TRPV4 is a polymodal, calcium-permeable cation channel that has emerged as a potential therapeutic target in multiple conditions. TRPV4, expressed in the plasma membrane of a wide range of cell types, is a polymodal ion channel whose gating is controlled by multiple endogenous lipids, and exogenous stimuli including synthetic ligands, cell swelling, shear stress, moderate heat, and ultraviolet light. Human TRPV4 adopts a two-layered homotetrameric architecture where RhoA attaches to the bottom layer. RhoA appears to act as an auxiliary subunit, interacting with the ARD through three loops connecting AR2-AR3, AR3-AR4, AR4-AR5, and with the membrane bilayer through the prenylated C-terminal tail.

Particle subtraction followed by focused 3D classification of the transmembrane region and RhoA-bound cytoplasmic domain were performed, resulting in improved map qualities for these regions for model building. In our ligand-bound 3D cryo-EM reconstructions, we identified strong and unambiguous EM densities corresponding to GSK279 (antagonist), GSK101 (agonist), and 4α-PDD (agonist) located at a shared site within the cavity between the VSLD and the TRP domain (termed here the VSLD cavity). We functionally probed the interactions of GSK101 with TRPV4 by mutating amino acid residues within the GSK101 binding site using patch clamp recording on HEK293 cells expressing WT as well as mutant TRPV4. Mutations Y553A, N474A, and F524A significantly increased EC50 values of GSK101 for TRPV4, consistent with observations from the structural analysis. The GSK101 binding pose remained stable during the simulations, supporting its accuracy. However, in the GSK101-bound open state, the SF and the PHs move closer to enable cation coordination (the diagonal distance of G679 backbone carbonyl is 7.0 Å), which is consistent with previous mutagenesis studies. Meanwhile the pore-lining S6 helices rotate ~90°, thus changing the gate position (from M718 to I715) and the gate opening (the diagonal distance at I715 is 8.3 Å). This S6 rotation between the two states is due to the shift of the π-helix position on S6, resulting in a local secondary structure conversion between α- and π-helix along S6b, which is unique amongst the TRP channels. To validate the S6 gate position observed in the open-state structure, we performed Cd2+-dependent blocking of TRPV4. Among cysteine mutants near the S6 gate (I715C, A716C, L717C, and M718C), only I715C showed substantial inhibition of GSK101-elicited current by extracellular Cd2+, supporting the observation that I715 faces the ion permeation pathway in the TRPV4 open state.

>[4x]MADSSEGPRAGPGEVAELPGDESGTPGGEAFPLSSLANLFEGEDGSLSPSPADASRPAGPGDGRPNLRMKFQGAFRKGVPNPIDLLESTLYESSVVPGPKKAPMDSLFDYGTYRHHSSDNKRWRKKIIEKQPQSPKAPAPQPPPILKVFNRPILFDIVSRGSTADLDGLLPFLLTHKKRLTDEEFREPSTGKTCLPKALLNLSNGRNDTIPVLLDIAERTGNMREFINSPFRDIYYRGQTALHIAIERRCKHYVELLVAQGADVHAQARGRFFQPKDEGGYFYFGELPLSLAACTNQPHIVNYLTENPHKKADMRRQDSRGNTVLHALVAIADNTRENTKFVTKMYDLLLLKCARLFPDSNLEAVLNNDGLSPLMMAAKTGKIGIFQHIIRREVTDEDTRHLSRKFKDWAYGPVYSSLYDLSSLDTCGEEASVLEILVYNSKIENRHEMLAVEPINELLRDKWRKFGAVSFYINVVSYLCAMVIFTLTAYYQPLEGTPPYPYRTTVDYLRLAGEVITLFTGVLFFFTNIKDLFMKKCPGVNSLFIDGSFQLLYFIYSVLVIVSAALYLAGIEAYLAVMVFALVLGWMNALYFTRGLKLTGTYSIMIQKILFKDLFRFLLVYLLFMIGYASALVSLLNPCANMKVCNEDQTNCTVPTYPSCRDSETFSTFLLDLFKLTIGMGDLEMLSSTKYPVVFIILLVTYIILTFVLLLNMLIALMGETVGQVSKESKHIWKLQWATTILDIERSFPVFLRKAFRSGEMVTVGKSSDGTPDRRWCFRVDEVNWSHWNQNLGIINEDPGKNETYQYYGFSHTVGRLRRDRWSSVVPRVVELNKNSNPDEVVVPLDSMGNPRCDGHQQGYPRKWRTDDAPLENSLEVLFQGPDYKDDDDKAHHHHHHHHHH>MGVVNVPSNGREKFKKNWKFCVGTGRLGLALQKEYLDHLKLVQEKIGFRYIRGHGLLSDDVGIYREVEIDGEMKPFYNFTYIDRIVDSYLALNIRPFIEFGFMPKALASGDQTVFYWKGNVTPPKDYNKWRDLIVAVVSHFIERYGIEEVRTWLFEVWNEPNLVNFWKDANKQEYFKLYEVTARAVKSVDPHLQVGGPAICGGSDEWITDFLHFCAERRVPVDFVSRHAYTSKAPHKKTFEYYYQELEPPEDMLEQFKTVRALIRQSPFPHLPLHITEYNTSYSPINPVHDTALNAAYIARILSEGGDYVDSFSYWTFSDVFEEMDVPKALFHGGFGLVALHSIPKPTFHAFTFFNALGDELLYRDGEMIVTRRKDGSIAAVLW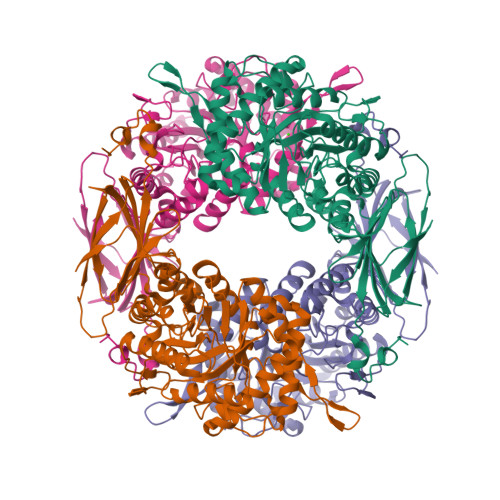NLVMEKGEGLTKEVQLVIPVSESAVFIKRQIVNEQYGNAWRVWKQMGRPRFPSRQAVETLRQVAQPHVMTEQRRATDGVIHLSIVLSKNEVTLIEIEQVRDETSTYVGLDDGEITSYSS[8x]> MKTEWPELVGKAVAAAKKVILQDKPEA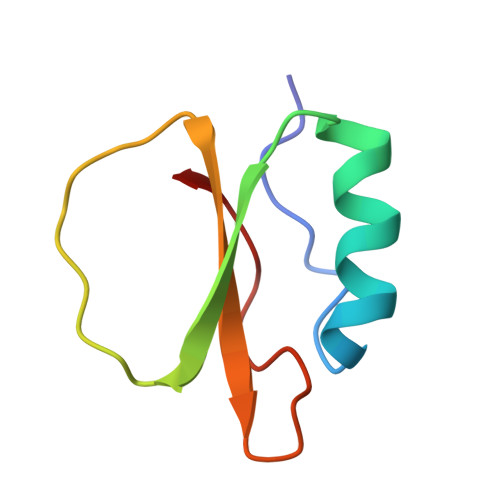QIIVLPVGTIVTMEYRIDRVRLFVDKLDNIAQVPRVG>MFDTKIA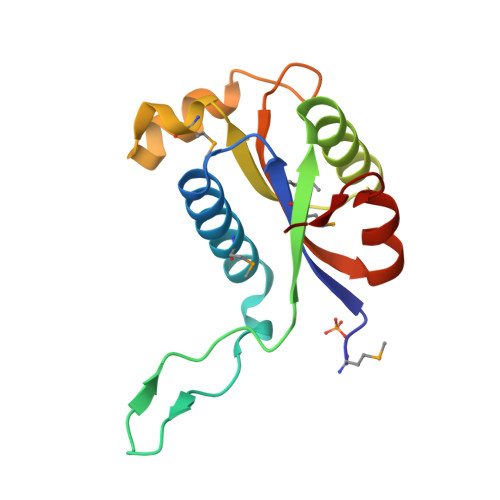VILRDDLAVWQKLNVTAFLMSGIVAQTGEIIGEPYRDGAGNVYNPLSIQPIVVMATDQEALRKIHQRSLERDITTSLYIEEMFATGHDAANRQVFSHFSPDTAKVVGMALRADRKIVDKITKGAKLHA[2x]> MERYENLFAQLNDRREGAFVPFVTLGDPGIEQSLKIIDTLIDAGADALELGVPFSDPLADGPTIQNANLRAFAAGVTPAQCFEMLAIIREKHPTIPIGLLMYANLVFNNGIDAFYARCEQVGVDSVLVADVPVEESAPFRQAALRHNIAPIFICPPNADDDLLRQVASYGRGYTYLLSR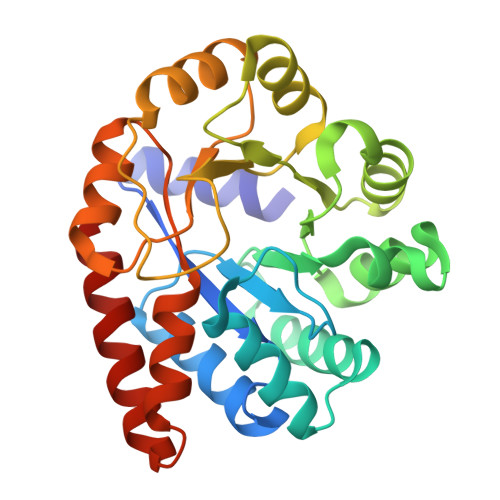SGVTGAENRGALPLHHLIEKLKEYHAAPALQGFGISSPEQVSAAVRAGAAGAISGSAIVKIIEKNLASPKQMLAELRSFVSAMKAASRA> ENLMQVYQQARLSNPELRKSAADRDAAFEKINEARSPLLPQLGLGADYTYSNGYRDANGINSNATSASLQLTQSIFDMSKWRALTLQEKAAGIQDVTYQTDQQTLILNTATAYFNVLNAIDVLSYTQAQKEAIYRQLDQTTQRFNVGLVAITDVQNARAQYDTVLANELTARNNLDNAVEQLRQITGNYYPELAALNVENFKTDKPQPVNALLKEAEKRNLSLLQARLSQDLAREQIRQAQDGHLPTLDLTASTGISDTSYSGSKTRGAAGTQYDDSNMGQNKVGLSFSLPIYQGGMVNSQVKQA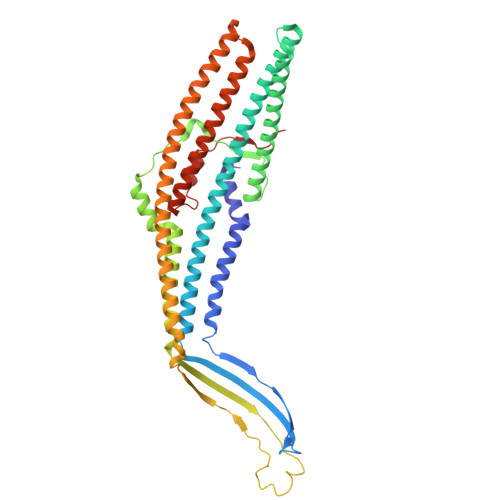QYNFVGASEQLESAHRSVVQTVRSSFNNINASISSINAYKQAVVSAQSSLDAMEAGYSVGTRTIVDVLDATTTLYNAKQELANARYNYLINQLNIKSALGTLNEQDLLALNNALSKPVSTNPE>GSHMTQSNLLPKTFRTKSGKEISIALGTGTKWKQAQTINDVSTELVDNILLGLKLGFRHIDTAEAYNTQKEVGEALKRTDVPREDIWVTTKYSPGWGSIKAYSKSPSDSIDKALAQLGVDYVDLFLIHSPFFTTEQTHGYTLEQAWEALVEAKKAGKVREIGISNAAIPHLEKLFAASPSPEYYPVVNQIEFHPFLQNQSKNIVRFCQEHGILVEAFSPLAPLARVETNALAETLKRLAEKYKKTEAQVLLRYTLQRGILPVTTSSKESRLKESLNLFDFELTDEEVNE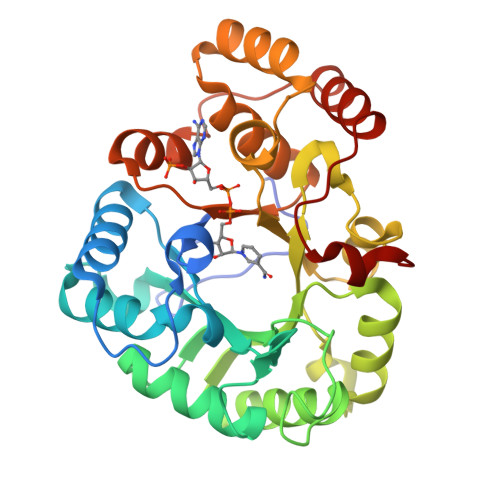INKIGDANPYRAFFHEQFKDL[2x]> PGDPQICPKRCVCQILSPNLATLCAKKGLLFVPPNI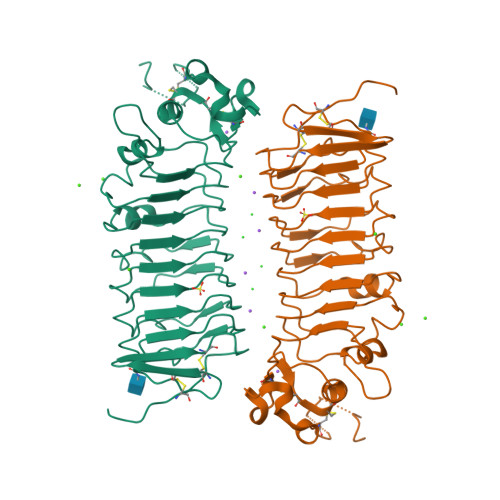DRRTVELRLADNFVTNIKRKDFANMTSLVDLTLSRNTISFITPHAFADLRNLRALHLNSNRLTKITNDMFSGLSNLHHLILNNNQLTLISSTAFDDVFALEELDLSYNNLETIPWDAVEKMVSLHTLSLDHNMIDNIPKGTFSHLHKMTRLDVTSNKLQKLPPDPLFQRAQVLATSGIISPSTFALSFGGNPLHCNCELLWLRRLSREDDLETCASPPLLTGRYFWSIPEEEFLCEPPLITRHTHEMRVLEGQRATLRCKARGDPEPAIHWISPEGKLISNATRSLVYDNGTLDILITTVKDTGAFTCIASNPAGEATQIVDLHIIAAAHHHHHH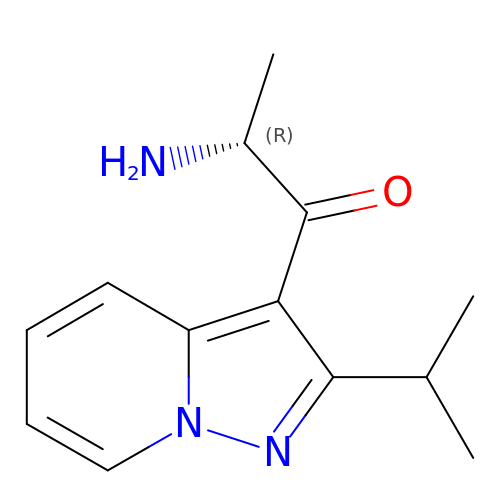(2R)-2-amino-1-[2-(1-methylethyl)pyrazolo[1,5-a]pyridin-3-yl]propan-1-one | C13 H17 N3 O | JLKPIOQFGACSJO-SECBINFHSA-N>MGVQPPNFSWVLPGRLAGLALPRLPA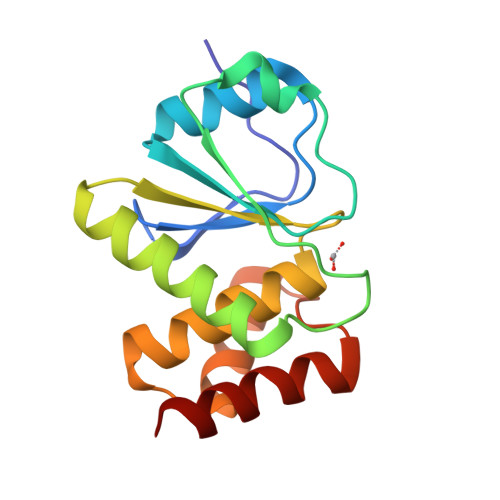HYQFLLDLGVRHLVSLTERGPPHSDSCPGLTLHRLRIPDFCPPAPDQIDRFVQIVDEANARGEAVGVHCALGFGRTGTMLACYLVKERGLAAGDAIAEIRRLRPGSIETYEQEKAVFQFYQRTK[2x]> GEVASVPLTNYLDSQYFGKIYLGTPPQEFTVLFDTGSSDFWVPSIYCKSNACKNHQRFDPRKSSTFQNLGKPLSIHYGTGSMQGILGYDTVTVSNIVDIQQTVGLSTQEPGDVFTYAEFDGILGMAYPSLASEYSIPVFDNMMNRHLVAQDLFSVYMDRNGQESMLTLGAIDPSYYTGSLHWVPVTVQQYWQFTVDSVTISGVVVACEGGCQAILDTGTSKLVGPSSDILNIQQAIGATQNQYGEFDIDCDNLSYMPTVVFEINGKMYPLTPSAYTSQDQGFCTSGFQSENHSQKWILGDVFIREYYSVFDRANNLVGLAKAI

Bovine and camel chymosin are aspartic peptidases that are used industrially in cheese production. They cleave the Phe105-Met106 bond of the milk protein κ-casein, releasing its predominantly negatively charged C-terminus, which leads to the separation of the milk into curds and whey. Despite having 85% sequence identity, camel chymosin shows a 70% higher milk-clotting activity than bovine chymosin towards bovine milk. The substrate-binding cleft and active site are located at the interface of the two domains.

Natural bovine chymosin is found in two isoforms, A and B, which differ at residue 244, which is an Asp in the A form and a Gly in the B form. It is the B form that is used in the investigations described in this paper, as it is commercially available in large quantities at high purity; it is referred to as ‘bovine chymosin’. Based on X-ray synchrotron-radiation data, the structure of bovine chymosin has been redetermined to 1.8 Å resolution. The structure of bovine chymosin does not differ from the three structures determined previously and can be superimposed with the earlier structures with an r.m.s.d. of 0.39 ± 0.02 Å (comparing 1733 atoms on average). In both the present structure of bovine chymosin and those determined by Gilliland et al., Strop et al., Newman et al. and Groves et al., the N-terminus is visible and forms one of the strands in an antiparallel β-sheet as in other aspartic peptidases such as porcine pepsin. In bovine chymosin the β-strand is formed by residues 4–6, with Ala4 and Val6 forming hydrogen bonds to Leu168 and Leu166, respectively. A prominent secondary structure in bovine chymosin is the central six-stranded antiparallel β-­sheet at the ‘bottom’ of the active site, which links and stabilizes the relative orientation of the two domains in the structure. The N-terminus of bovine chymosin forms one of the strands in this sheet. The engagement of residues 4–6 in the β-sheet in bovine chymosin keeps the N-terminal loop in a conformation in which it forms part of the binding cleft; in camel chymosin the same residues point towards the active site. The chloride ions in bovine chymosin and the sulfate ions in camel chymosin are located adjacent to these patches, demonstrating the impact of the positively charged patches of the structures. Previous studies of bovine chymosin have identified a positively charged patch on the N-terminal domain and a negatively charged patch on the C-terminal domain adjacent to the substrate-binding cleft; these patches were suggested to influence the interaction with κ-casein.>MAEEGTRSEAADAATQARQLPDSRNIFVSHRFPERQVDLGEVVMNFAEAGSPDNPALLLLPEQTGSWWSYEPVMGLLAENFHVFAVDIRGQGRSTWTPRRYSLDNFGNDLVRFIALVIKRPVVVAGNSSGGLLAAWLSAYAMPGQIRAALCEDAPFFASELVPAYGHSVLQAAGPAFELYRDFLGDQWSIGDWKGFVEAAKASPAKAMQLFPTPDEAPQNLKEYDPEWGRAFFEGTVALHCPHDRMLSQVKTPILITHHARTIDPETGELLGALSDLQAEHAQDIIRSAGVRVDYQSHPDALHMMHLFDPARYAEILTSWSATLPANDHHHHHH[4x]

Zearalenone (ZEN) is a mycoestrogenic polyketide produced by Fusarium graminearum and other phytopathogenic members of the genus Fusarium. ZenA cleaves zearalenone [ZEN, (S,E)-14,16-dihydroxy-3-methyl-3,4,5,6,9,10-hexahydro-1H-benzo[c][1]oxacyclotetradecine-1,7(8H)-dione] to hydrolyzed zearalenone [HZEN, (S,E)-2,4-dihydroxy-6-(10-hydroxy-6-oxoundec-1-en-1-yl)benzoic acid], which decarboxylates spontaneously to decarboxylated hydrolyzed zearalenone [DHZEN, (S,E)-1-(3,5-dihydroxyphenyl)-10-hydroxyundec-1-en-6-one]. Furthermore, we report site-directed mutagenesis as well as structural analysis of the dimeric ZenARe of R. erythropolis and the more thermostable, tetrameric ZenAScfl of Streptomyces coelicoflavus with and without bound ligands. The X-ray crystal structures not only revealed canonical features of α/β hydrolases with a cap domain including a Ser-His-Asp catalytic triad but also unusual features including an uncommon oxyanion hole motif and a peripheral, short antiparallel β-sheet involved in tetramer interactions.

As HZEN was found bound at the active site of ZenAScfl H286Y after cocrystallization with ZEN, cocrystallization of wild-type, active ZenARe with ZEN was also attempted. The RMSD compared with the structure without ligand was 0.147 Å (over 251 Cα), and compared with the structure with bound ZLAEN, it was 0.131 Å (over 276 Cα). The structure showed again that the position of the resorcylic acid moiety was well-defined. The lactone ester bond was cleaved, and the aliphatic hydroxy ketone moiety appeared flexible. Residues interacting with the bound ligand were positioned as in the closed conformation of ZenARe with bound ZLAEN. The carboxylate atom O12 was at a distance of 3.1 and 3.1 Å from the N of oxyanion hole residue I and the amide N of oxyanion hole residue II, respectively. The nucleophilic serine Ser-112 appeared in the same orientation as in the structure with ZLAEN bound, with its OG at a distance of 2.7 Å from C12 of the carboxylic acid group. Nonpolar interactions with HZEN were again formed by the residues from the cap domain, with a π–π stacking interaction mediated by Phe-177. Additionally, the catalytic His-303 showed involvement in a weak electrostatic interaction with C12 of the carboxylic acid group of HZEN at 5.1 Å distance.> MSLRTLVAGVDTSTQSCKVRVTDAETGELVRFGQAKHPNGTSVDPSYWWSAFQEAAEQAGGLDDVSALAVGGQQHGMVILDNQGNVIRDAMLWNDTSSAPQAAALIEKLGAAPAQDGEPEDPIARGKQRWVKAVGSSPVASYTLTKVAWVAENEPENVKKIAAICLPHDWLSWRIAGYGPVAEGEDAHLEALFTDRSDASGTIYYDAASNEYRRDLIAMVLEAAEGAKAAQSHAEAIVLPTVLGPRDAAPVKADPAIAGKNVEGGCLLAPGGGDNAMASLGLGMAVGDVSISLGTSGVAAAISENPTYDLTGAVSGFADCTGHYLPLACTINGSRILDAGRAALGVDYDELAKLAFASKPGANGITLVPYFDGERTPNRPNATATFSGMTLANTTRENLARAFVEGLLCSQRDCLELIRSLGASITRILLIGGGAKSEAIRTLAPSILGMDVTRPATDEYVAIGAARQAAWVLSGETEPPAWQLTIDGVETGEPTEAVY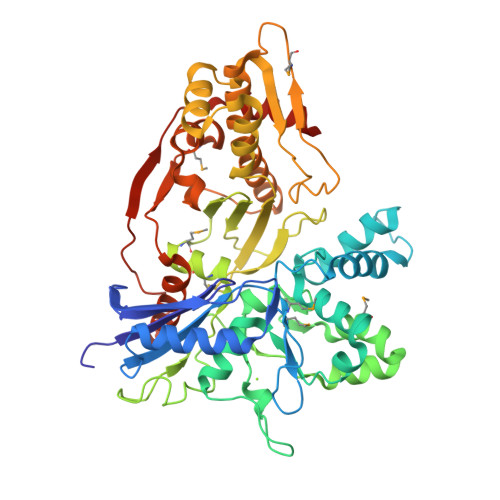EAYAKARGEGHHHHHH>[5x]GSNGMSQLPAPVSVESSWRYIDTQGQIHGP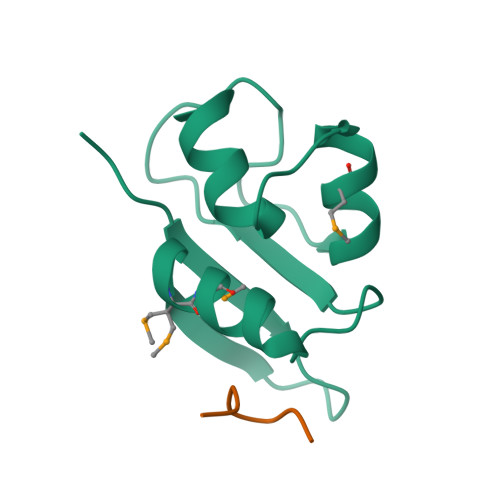FTTQMMSQWYIGGYFASTLQISRLGSTPETLGINDIFITLGELMTKLEKYDTDPFTTFDKLHVQTTSSDS;>SSIAPPPGLSG[5x]>SNTQAERSIIGMIDMFHKYTRRDDKIDKPSLLTMMKENFPNFLSACDKKGTNYLADVFEKKDKNEDKKIDFSEFLSLLGDIATDYHK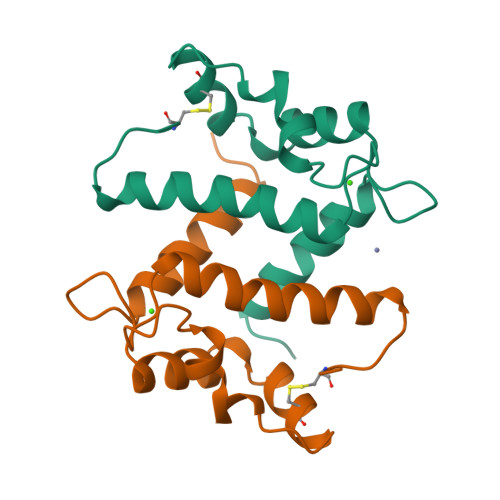QSHGAAPCSGGSQ[2x]>[12x]GHMEQTHRAIFRFVPRHEDELELEVDDPLLVELQAEDYWAEAYNMRT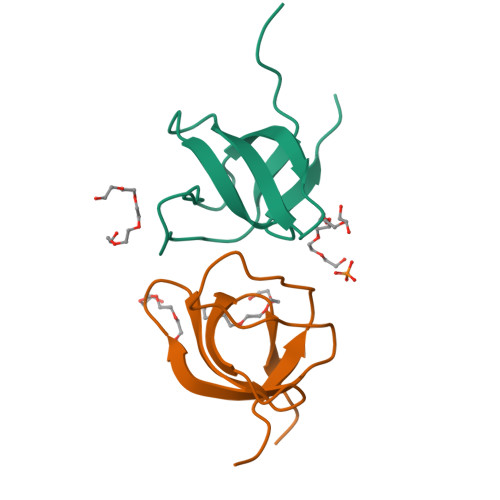GARGVFPAYYAIEVTK> NHATAPMTRAPAPEYVPEAPRHS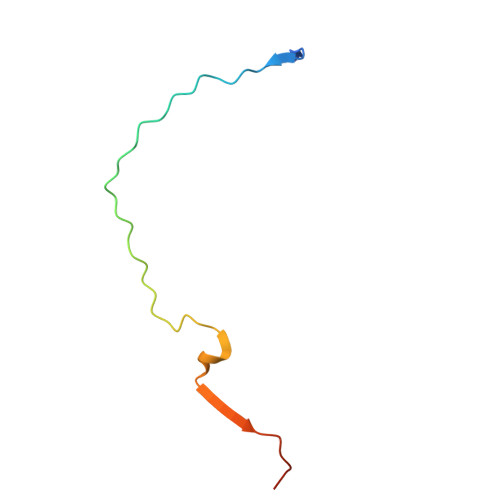DWQRPTFAFEGKGAAGGHTATHHASAAPARPQPVE> GAPTKVTFGDDTVIEVQGYKSVNITFELDERIDKVLNEKCSAYTVELGTEVNEFACVVADAVIKTLQPVSELLTPLGIDLDEWSMATYYLFDESGEFK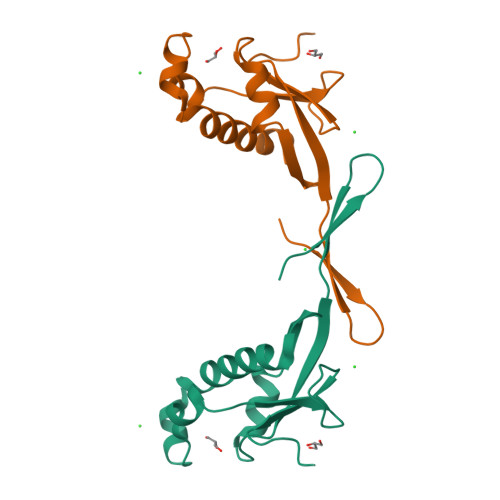LASHMYCSFYPPDE>SDNTRTLPDRENSCPGLLLLLLPIMKTAIALLPFLGAATAFVTPMSKTSMARGRSLQMSFDDEAGAIQWFPPSPGYWDPLGFVADGDTEKFSKYRAIEIKHGRVAMLGALDYFIKTPSGWHLPGKLGDVDIDSIPVGLGAIKAVPPLGWVQILLFASALEFLAPQKEDQPPGAVQPATPSFEQPGTLEYQTKEINNGRLAMIALAGLWLGELASGGTDPIVAFKTWVGI[2x];>[2x]MVAKSAALVVMGLSMASAFLAPTPNNRASAQAPMKMAKSAATKEFPFDDQPGGVKWFPSSAPYWDPLGFT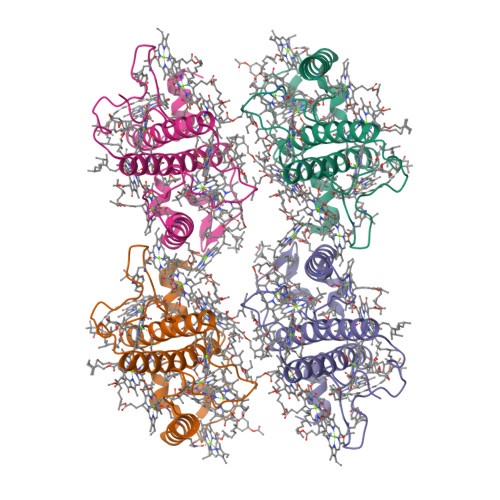NEKTEDEYWRIAHGEIKNGRLAMLAVTHYFVVGSGLRFPFKFGSVSTADVPLGLGAIKALPWAVWLQIAAFCLVLEVLTENPGFGERVPGRVPGNLQPDTPSFNAPGDLEIRTKELNNARLAMISIWGLWVGEIASGGVDPFTSFANWLKL> MTAILIQSEEYVDLTFKLRGAPIPLDNGYLTYAALSRICPPLHELKSIGIHPIAGIPTRNNLLELTAQSRLKIRIYHQQIPLIYPYLAGQAFHIGQNFYQLDIPDYKPLISSESVYSRLVIIKGFQDSTNFIEAVQRQMDNLGIQGKI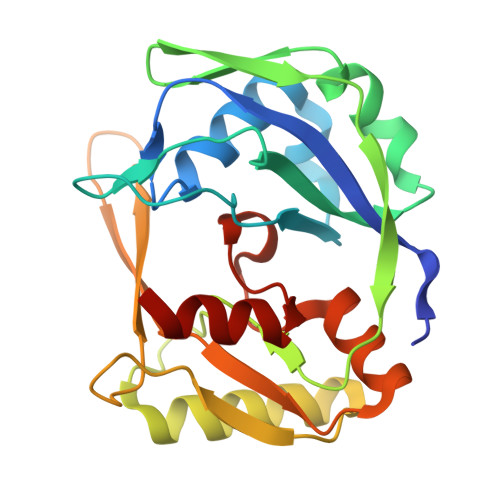ELLTRQDGTPQRRQLTINKEGKQFKVRGFGVKISELNPEDSLTLQEQGIGGKRKMMCGIFVPATRSKEEEET> SSLDDKPQFPGASAEFIDKLEFIQPNVISGIPIYRVMDRQGQIINPSEDPHLPKEKVLKLYKSMTLLNTMDRILYESQRQGRISFYMTNYGEEGTHVGSAAALDNTDLVFGQYREAGVLMYRDYPLELFMAQCYGNISDLGKGRQMPVHYGCKERHFVTISSPLATQIPQAVGAAYAAKRANANRVVICYFGEGAASEGDAHAGFNFAATLECPIIFFCRNNGYAISTPTSEQYRGDGIAARGPGYGIMSIRVDGNDVFAVYNATKEARRRAVAENQPFLIEAMTYRIGHHETSDDSSAYRSVDEVNYWDKQDHPISRLRHYLLSQGWWDEEQEKAWRKQSRRKVMEAFEQAERKPKPNPNLLFSDVYQEMPAQLRKQQESLARHLQTYGEHYPLDHFDK;> VAHFTFQPDPEPREYGQTQKMNLFQSVTSALDNSLAKDPTAVIFGEDVAFGGVFRCTVGLRDKYGKDRVFNTPLCEQGIVGFGIGIAVTGATAIAEIQFADYIFPAFDQIVNEAAKYRYRSGDLFNCGSLTIRSPWGCVGHGALYHSQSPEAFFAHCPGIKVVIPRSPFQAKGLLLSCIEDKNPCIFFEPKILYRAAAEEVPIEPYNI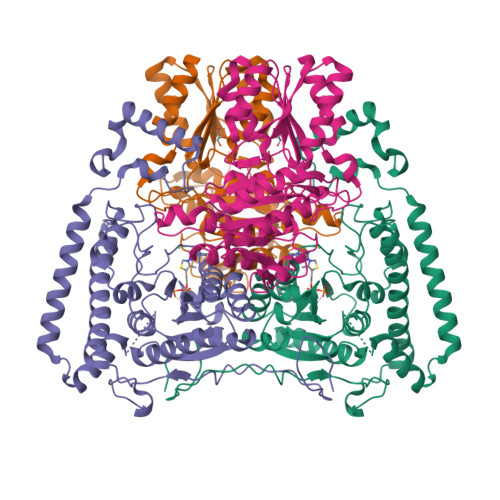PLSQAEVIQEGSDVTLVAWGTQVHVIREVASMAKEKLGVSCEVIDLRTIIPWDVDTICKSVIKTGRLLISHEAPLTGGFASEISSTVQEECFLNLEAPISRVCGYDTPFPHIFEPFYIPDKWKCYDALRKMINY> GGCGCACUGGCGCUGCGCCUUCGGGCGCCAAUCG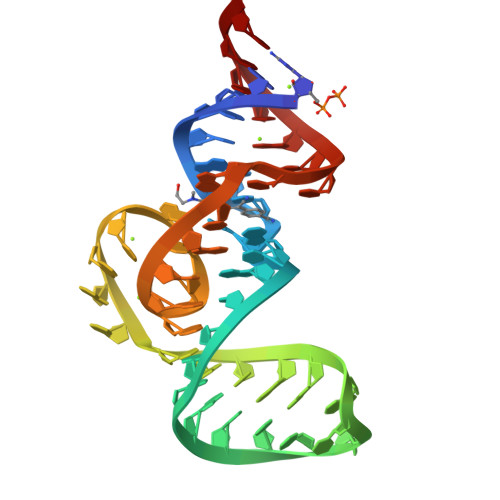UAGCGUGUCGGCGCC> SADAQSFLNRVCGVSAARLTPCGTGTSTDVVYRAFDIYNDKVAGFAKFLKTNCCRFQEKDEDDNLIDSYFVVKRHTFSNYQHEETIYNLLKDCPAVAKHDFFKFRIDGDMVPHISRQRLTKYTMADLVYALRHFDEGNCDTLKEILVTYNCCDDDYFNKKDWYDFVENPDILRVYANLGERVRQALLKTVQFCDAMRNAGIVGVLTLDNQDLNGNWYDFGDFIQTTPGSGVPVVDSYYSLLMPILTLTRALTAESHVDTDLTKPYIKWDLLKYDFTEERLKLFDRYFKYWDQTYHPNCVNCLDDRCILHCANFNVLFSTVFPPTSFGPLVRKIFVDGVPFVVSTGYHFRELGVVHNQDVNLHSSRLSFKELLVYAADPAMHAASGNLLLDKRTTCFSVAALTNNVAFQTVKPGNFNKDFYDFAVSKGFFKEGSSVELKHFFFAQDGNAAISDYDYYRYNLPTMCDIRQLLFVVEVVDKYFDCYDGGCINANQVIVNNLDKSAGFPFNKWGKARLYYDSMSYEDQDALFAYTKRNVIPTITQMNLKYAISAKNRARTVAGVSICSTMTNRQFHQKLLKSIAATRGATVVIGTSKFYGGWHNMLKTVYSDVENPHLMGWDYPKCDRAMPNMLRIMASLVLARKHTTCCSLSHRFYRLANECAQVLSEMVMCGGSLYVKPGGTSSGDATTAYANSVFNICQAVTANVNALLSTDGNKIADKYVRNLQHRLYECLYRNRDVDTDFVNEFYAYLRKHFSMMILSDDAVVCFNSTYASQGLVASIKNFKSVLYYQNNVFMSEAKCWTETDLTKGPHEFCSQHTMLVKQGDDYVYLPYPDPSRILGAGCFVDDIVKTDGTLMIERFVSLAIDAYPLTKHPNQEYADVFHLYLQYIRKLHDELTGHMLDMYSVMLTNDNTSRYWEPEFYEAMYTPHTVLQ;>[2x]MGSSHHHHHHENLYFQSNAAIASEFSSLPSYAAFATAQEAY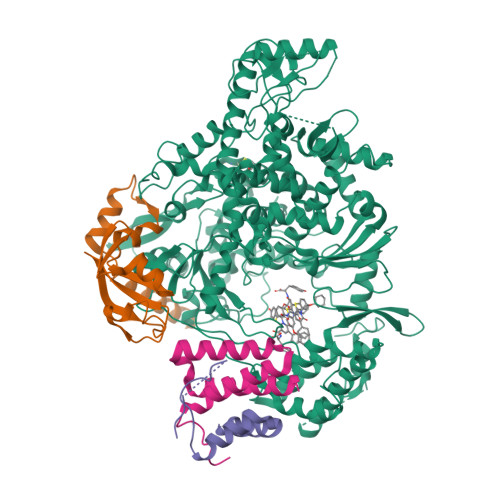EQAVANGDSEVVLKKLKKSLNVAKSEFDRDAAMQRKLEKMADQAMTQMYKQARSEDKRAKVTSAMQTMLFTMLRKLDNDALNNIINNARDGCVPLNIIPLTTAAKLMVVIPDYNTYKNTCDGTTFTYASALWEIQQVVDADSKIVQLSEISMDNSPNLAWPLIVTALRANSAVKLQ;> SNASKMSDVKCTSVVLLSVLQQLRVESSSKLWAQCVQLHNDILLAKDTTEAFEKMVSLLSVLLSMQGAVDINKLCEEMLDNRAT1-[4-chloranyl-3-(trifluoromethyl)phenyl]-1,2,3-triazole | C9 H5 Cl F3 N3 | 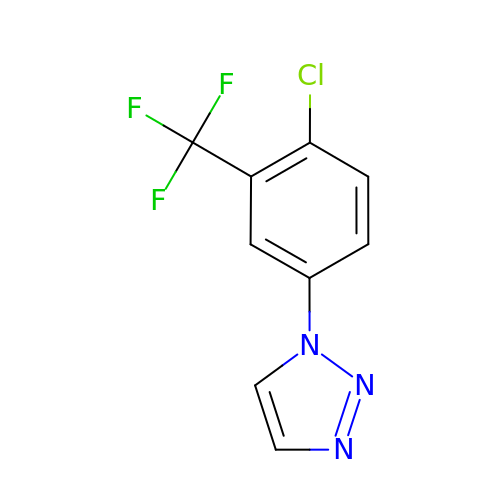SYIRPQOOLRXDHA-UHFFFAOYSA-N>[2x]GMGK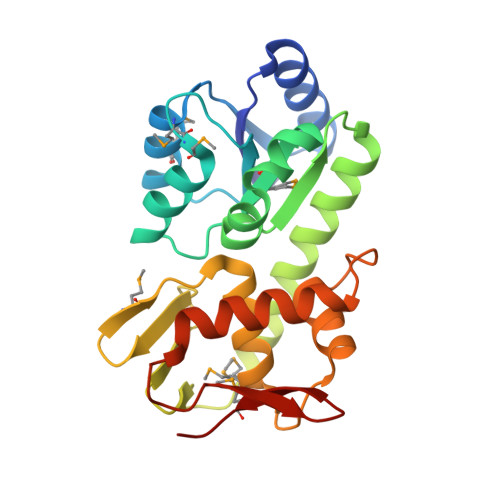RILLLEKERNLAHFLSLELQKEQYRVDLVEEGQKALSMALQTDYDLILLNVNLGDMMAQDFAEKLSRTKPASVIMILDHWEDLQEELEVVQRFAVSYIYKPVLIENLVARISAIFRGRDFIDQHSSLMKVPRTYRNLRIDVEHHTVYRGEEMIALTRREYDLLATLMGSKKVLTREQLLESVWKYESATETNIVDVYIRYLRSKLDVKGQKSYIKTVRGVGYTMQEG>[3x]EVNEKAPAQA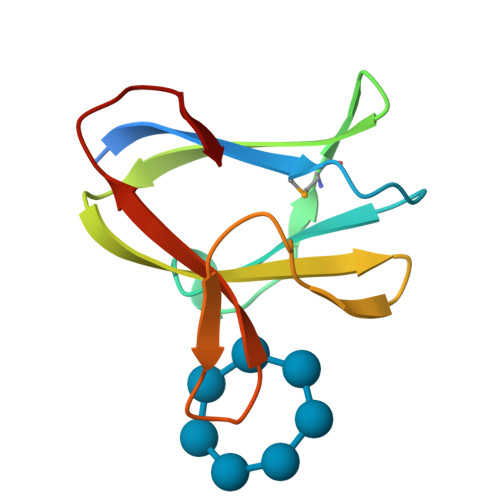RPTVFRWTGGGKEVYLSGSFNNWSKLPMTRSQNNFVAILDLPEGEHQYKFFVDGQWTHDPSEPIVTSQLGTVNNIIQVKKTDFEVF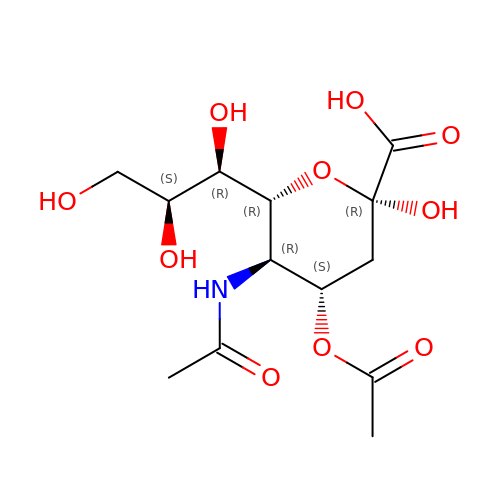4-O-acetyl-5-acetamido-3,5-dideoxy-L-glycero-alpha-D-galacto-non-2-ulopyranosonic acid | C13 H21 N O10 | LVBIMVQYUKOENY-DQBXORCPSA-N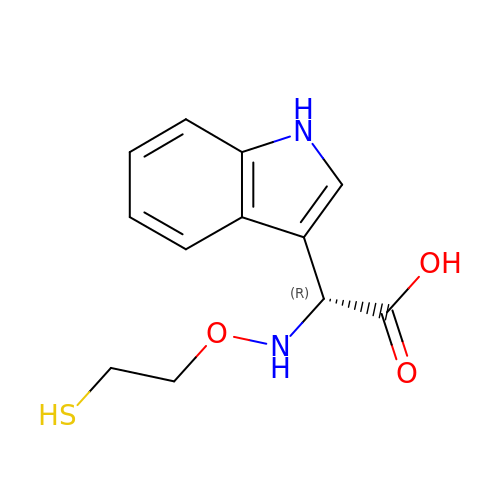(1H-INDOL-3-YL)-(2-MERCAPTO-ETHOXYIMINO)-ACETIC ACID | C12 H14 N2 O3 S | FJAWIBGKKKXXAL-LLVKDONJSA-N> MINVSGFGTGIVIVS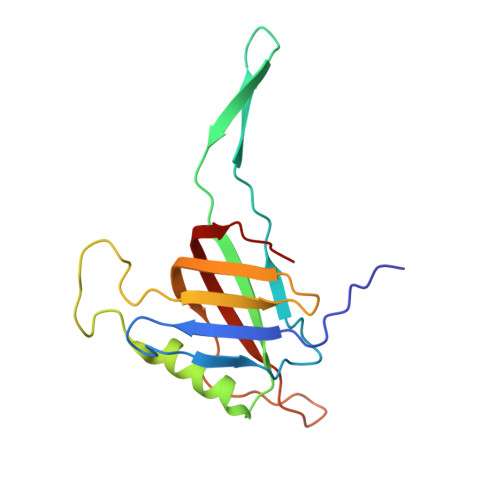ASSFPMGFSLSKFADDESPISSKELEPFGYEMLYDGGLFAFDKAAPLEVSVSVIAGSEDDINLRILLNSKKGSFRFLPGIIPDMTTLVATLPDGGRTVLSNGTILKGPAIDTIQNTGRRKGNTYTFVFGSYLGAQTA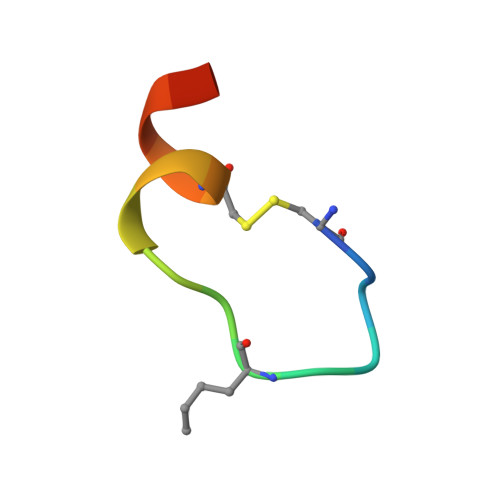> CDIHVLWEWDCFEKLX> RSEVIASGRLEKCVVDGVTEELDCQEKVVVTLTVGNGQSLQTEALEFSLSCLNSPDGRCPCSCSAADPTCACRDLAAPLRVSLTKSPLWASYPLQ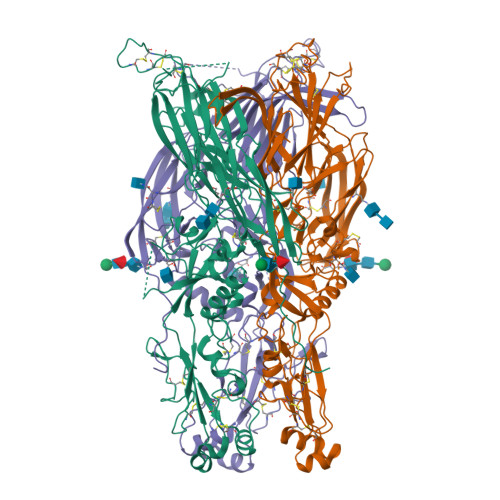YLSSFNWKPLEVILRPSNKVCKDGDWEDSPTCGWFSQGGVRVADSQGFCCECSSSQVWDDTFGSSKERTRANLDCDFWSDPLDILIGRKPVSAHCLTFDPQWYSGYELGAASLQFEIAITVEVPTAPSPTTATTSATPRTNNSSSANSTNSTNSPAPQFLSPPAPSTREVLHLGPSVPLASSASRLLSAKLLGDLAMYTQLPAISNQVLMVPQPPAAAAATGSPLDATLATNRSAWMLLDKTMLSMDGLACDKVGTGFSAFRYQPSGCGRAPQACLSGQLKDLWEADLARIADGRVPLYMITRFTGGSDTTLQSFSGGPLSFALPVTSHSQSLVTLSVAADGVRLVTNRSPGKITGAAVCRFAGTSCGGFEAVAARGYIYVNITNTGRLDSDYTLTVSNCSSNVRPIEARTLAVRAGSAASLDPPMELYVEDQAAAAARTCTVSLYDSVGAVTDSLTLSFYTNATQLVVKPSGGYNGGPFEDDDDK>ADPQKLDDVDPLVTTNFGKIRGIKKELNNEILGPVIQFLGVPYAAPPTGEHRFQPPEPPSPWSDIRNATQFAPVCPQNIIDGRLPEVMLPVWFTNNLDVVSSYVQDQSEDCLYLNIYVPTEDDIRDSGGPKPVMVYIHGGSYMEGTGNLYDGSVLASYGNVIVITVNYRLGVLGFLSTGDQAAKGNYGLLDLIQALRWTSENIGFFGGDPLRITVFGSGAGGSCVNLLTLSHYSEKGLFQRAIAQSGTALSSWAVSFQPAKYARILATKVGCNVSDTVELVECLQKKPYKELVDQDVQPARYHIAFGPVIDGDV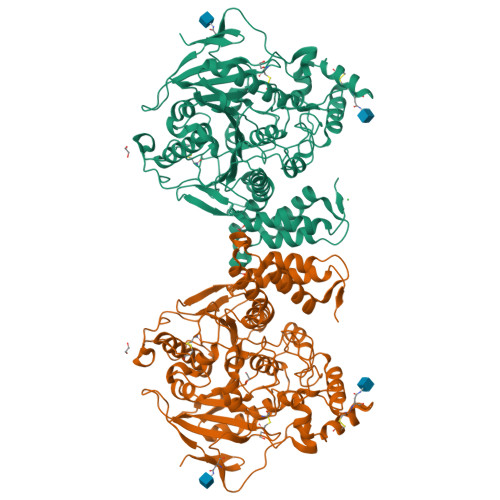IPDDPQILMEQGEFLNYDIMLGVNQGEGLKFVENIVDSDDGVSASDFDFAVSNFVDNLYGYPEGKDVLRETIKFMYTDWADRHNPETRRKTLLALFTDHQWVAPAVATADLHSNFGSPTYFYAFYHHCQTDQVPAWADAAHGDEVPYVLGIPMIGPTELFPCNFSKNDVMLSAVVMTYWTNFAKTGDPNQPVPQDTKFIHTKPNRFEEVAWTRYSQKDQLYLHIGLKPRVKEHYRANKVNLWLELVPHLHNLNDHHHHHH[4x]> GIDPFTARTQVTRAVSEVSA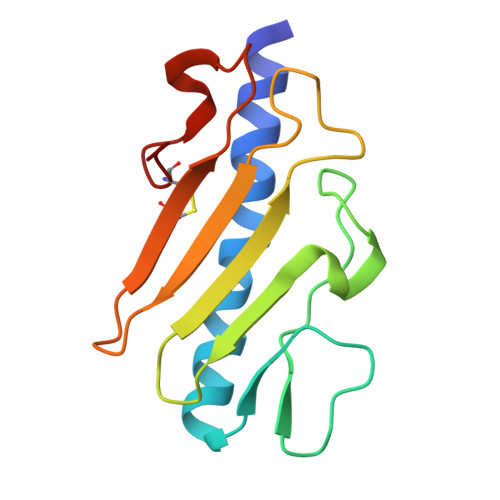LKTAAESAILEGKEIVSSATPKDTQYDIGFTESTLLDGSGKSQIQVTDNQDGTVELVATLGKSSGSAIKGAVITVSRKNDGVWNCKITKTPTAWKPNYAPANCPKS> MHRVMGIETEYGISVPHQPNANAMAASSQVVNAYAPIGAPAQRQARWDFEEENPLRDARGFEVAREAADPSQLTDEDLGLANVILTNGARLYVDHAHPEYSTPEVTNPRDAVLWDKAGERIMAEAARRAADLPMGWTIQLYKNNTDNKGASYGCHENYLMNRSTPFADIVRHLIPFFVTRQVFCGAGRVGIGADGRGEGFQLSQRADFFEVEVGLETTLKRPIINTRDEPHA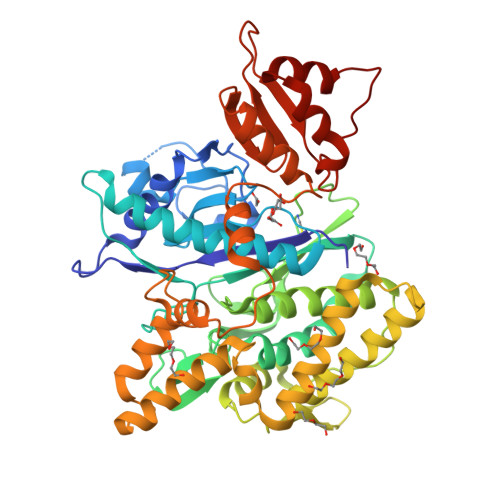DPEKYRRLHVIIGDANMSEIATYLKLGTTALVLAMIEDGFLSQDFSVESPVGALRAVSHDPTLRYQLRLHDGRRLTAVQLQMEYLEQARKYVEDRFGTDVDDMTRDVLDRWETTLVRLADDPMQLSRDLDWVAKLSILEGYRQRENLPWSAHKLQLVDLQYHDVRPDRGLYNRLVARGRMNLLVDEAAVRTAMHEPPNDTRAYFRGRCLAKFGAEIAAASWDSVIFDLPGRDSLQRVPTLEPLRGTRAHVGDLLDRCRSATELVAALTGGENLYFQ>HHHHHHGSGSQSVQAKAEVKQQSESELKHYYNKPILERKNVTGFKYTDEGKHYLEVTVGQQHSRITLLGSDKDKFKDGENSNIDVFILREGDSRQATNYSIGGVTKSNSVQYIDYINTPILEIKKDNEDVLKDFYYISKEDISLKELDYRLRERAIKQHGLYSNGLK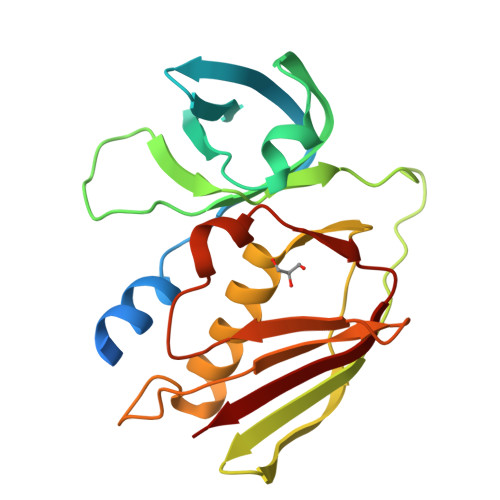QGQITITMNDGTTHTIDLSQKLEKERMGESIDGTKINKILVEMK[6x]>AVANSIVSSVAPGKEPGSLVCIQAKDGKVIGMGARVHCGPATV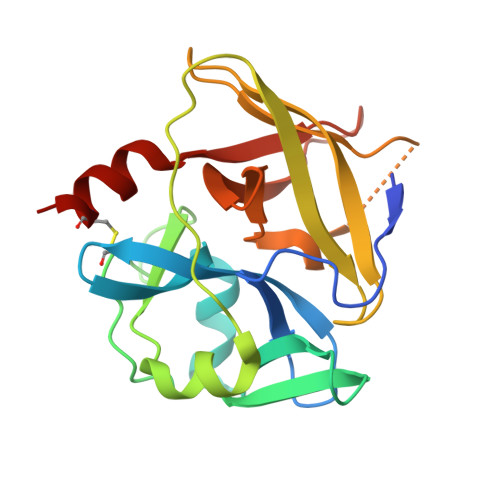LVTAGHVLKKGMIADLYLAKYSVSSKEGKRVLMDPTWKIEYGSLNKEADVISVQVPAAVWSRLGVTAARVRKPTVKVPVLAYGGEASGLLQSSQGFATPDGNMSVAHSCSTRPGWSGTPLYAGSDIVAIHRRWEDIGVKNLATNLSIFHANCESSE[2x]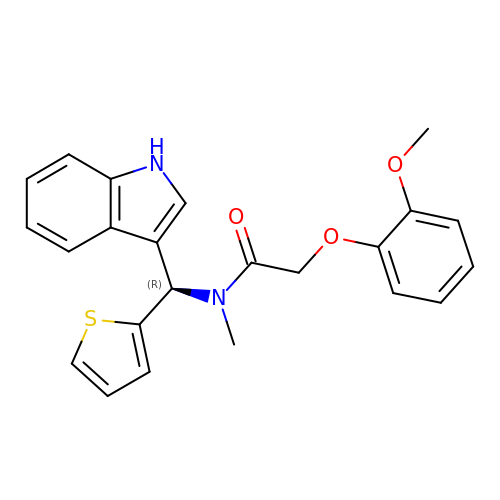N-[(R)-(1H-indol-3-yl)(thiophen-2-yl)methyl]-2-(2-methoxyphenoxy)-N-methylacetamide | C23 H22 N2 O3 S | UMXDHOYRZISANE-HSZRJFAPSA-N> TLRTSGELLQGIVRVYSKQATFLLTDIKDTLTKISMLVIFTDVLKSITKRE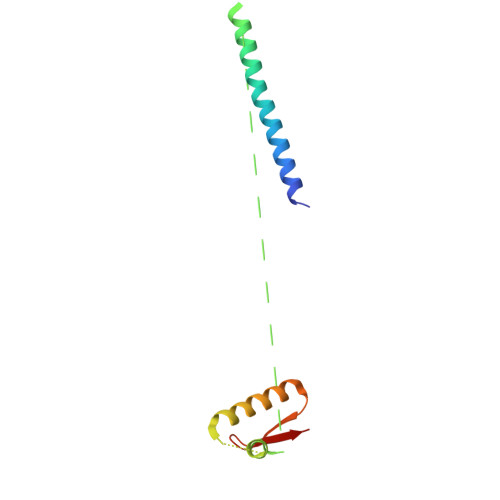ASRGFFDILSLATEGCIGLSQTEAFGNIKIDA> MIITLIAAMDKNRLIGRNNELPWHLPADLAHFKSITLGKPIVMGRRTFDSIGKPLPHRRNIVITQQKNLIIEGCDIFYSLDDALSALTKEPEVIIIGGARIFKEALPKADKMILTIINHSFEGDVYFPEWNDKEWKITSQIKHERD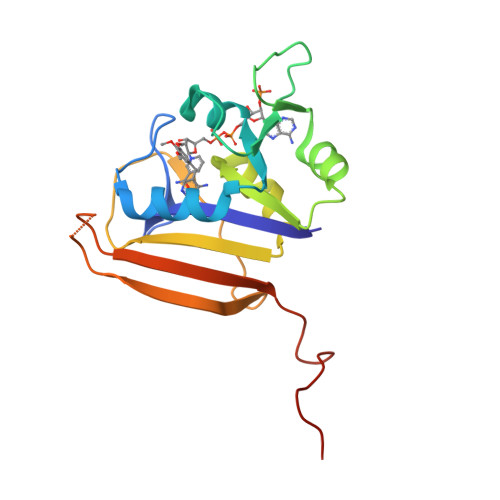EKNPYPFQFLELRRLENLYFQGHHHHHHHHHH> YAPSALVLTVGKGVSATTAAPERAVTLTCAPGPSGTHPAAGSACADLAAVGGDLNALTRGEDVGCPKV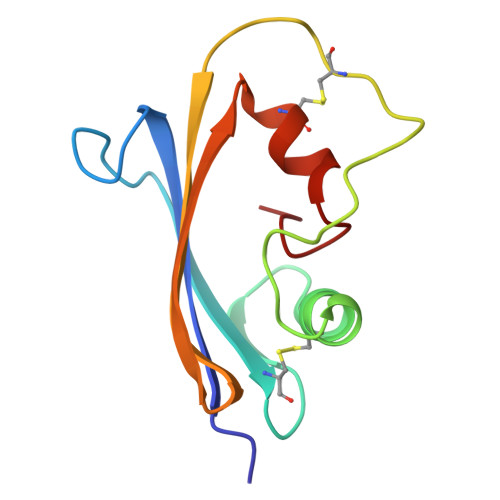YDPVLLTVDGVWQGKRVSYERVFSNECEMNAHGSSVFAF>[2x]MDEFEMIKRNTSEIISEEELREVLKKDEKSAQIGFEPSGKIHLGHYLQIKKMIDLQNAGFDIIILLADLHAYLNQKGELDEIRKIGDYNKKVFEAMGLKAKYVYGSTFQLDKDYTLNVYRLALKTTLKRARRSMELIAREDENPKVAEVIYPIMQVNA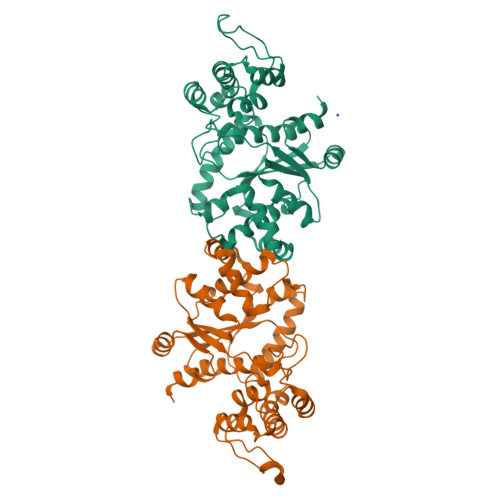IHYPGVDVAVGGMEQRKIHMLARELLPKKVVCIHNPVLTGLDGEGKMSSSKGNFIAVDDSPEEIRAKIKKAYCPAGVVEGNPIMEIAKYFLEYPLTIKRPEKFGGDLTVNSYEELESLFKNKELHPMDLKNAVAEELIKILEPIRKRLHHHHHH> MKKGHHHHHHGQKPKYQVRWKIIES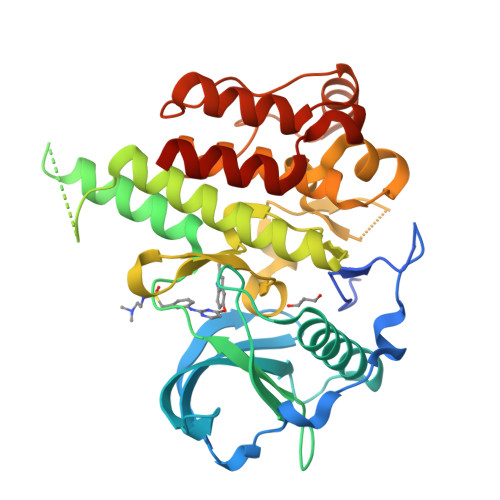YEGNSYTFIDPTQLPYNEKWEFPRNNLQFGKTLGAGAFGKVVEATAFGLGKEDAVLKVAVKMLKSTAHADEKEALMSELKIMSHLGQHENIVNLLGACTHGGPVLVITEYCTYGDLLNFLRRKAEAMLGPSLSPGQDPEGGVDYKNIHLEKLDKEDGRPLELRDLLHFSSQVAQGMAFLASKNCIHRDVAARNVLLTNGHVAKIGDFGLARDIMNDSNYIVKGNARLPVKWMAPESIFDSVYTVQSDVWSYGILLWEIFSLGLNPYPGILVNSKFYKLVKDGYQMAQPAFAPKNIYSIMQACWALEPTHRPTFQQITSFLQEQAQEDRR> KMKPFIFGAR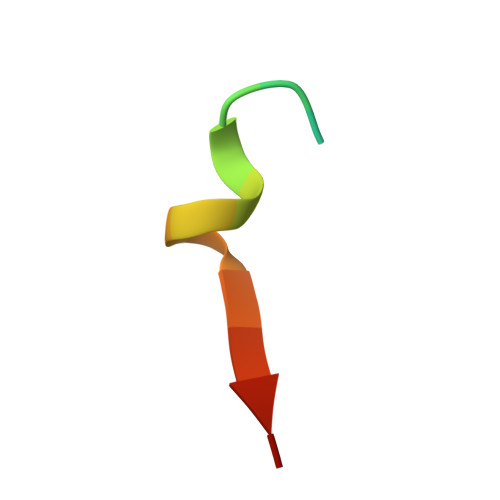NKVHIYX>[2x]GKESICLPFNFHSHRQHTCLDISPYGNEQVSRIACTSCEDNRILPTASDAMVAFINQTSNIMKNRNFYYGFCKSSELLKLS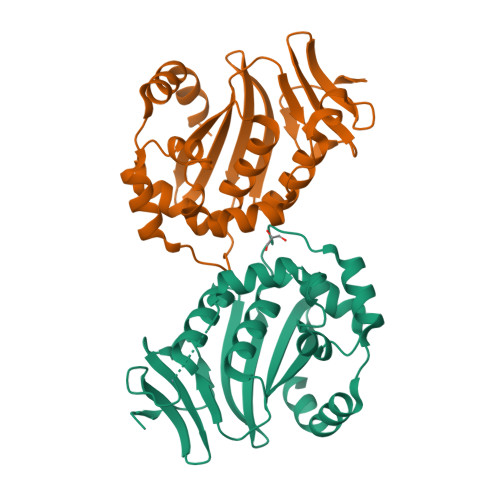TNQPPIFQIYYLLHAANHDIVPFMHAEDGRLHMHVIFENPDVHIPCDCITQMLTAAREDYSVTLNIVRDHVVISVLCHAVSASSVKIDVTILQRKIDEMDIPNDVSESFERYKELIQELCQS> MGSMEDITTLLSMTQPLKLRGFQKWDVFCNAVNNMMNNPLLPAHGKGVLVALRPVPGIRVEQALTLCRPNRTGDIMTIGGN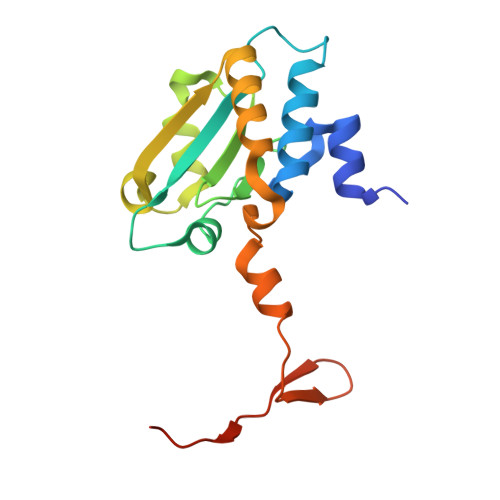RLVLFLSFCRINDLDTALNHIFPLPTGDIFSNRMVWFEDDQISAELVQMRLLAPEQWGMPLPLTQSSKPVINAEHDGRHWRRIPEPMRLLDDAVERSS>MAKKKKKKSFNTTRPTDPPVYPVTVPFLGHIVQFGKNPLEFMQRCKRDLKSGVFTISIGGQRVTIVGDPHEHSRFFSPRNEILSPREVYTIMTPVFGEGVAYAAPYPRMREQLNFLAEELTIAKFQNFVPAIQHEVRKFMAENWKEDEGVINLLEDCGAMIINTACQCLFGEDLRKRLNARHFAQLLSKMESSLIPAAVFMPWLLRLPLPQSARCREARAELQKILGEIIVAREKEEASKDNNTSDLLGGLLKAVYRDGTRMSLHEVCGMIVAAMFAGQHTSTITTSWSMLHLMHPKNKKWLDKLHKEIDEFPAQLNYDNVMDEMPFAERCVRESIRRD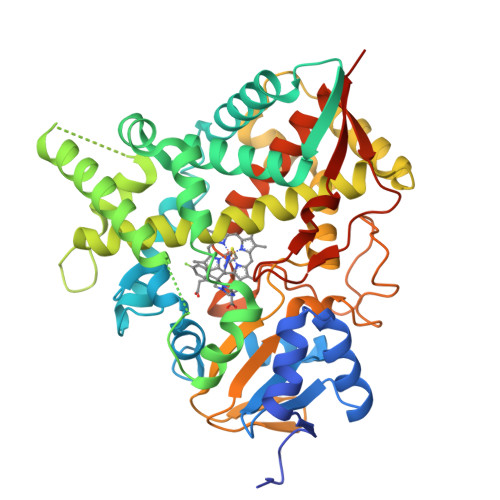PPLLMVMRMVKAEVKVGSYVVPKGDIIACSPLLSHHDEEAFPNPRLWDPERDEKVDGAFIGFGAGVHKCIGQKFALLQVKTILATAFREYDFQLLRDEVPDPDYHTMVVGPTLNQCLVKYTRKKKLPSHHHHHH[2x]>[2x]GKQLTILGSTGSIGCSTLDVVRHNPEHFRVVALVAGKNVTRMVEQCLEFSPRYAVMDDEASAKLLKTMLQQQGSRTEVLSGQQAACDMAALEDVDQVMAAIVGAAGLLPTLAAIRAGKTILLANKESLVTCGRLFMDAVKQSKA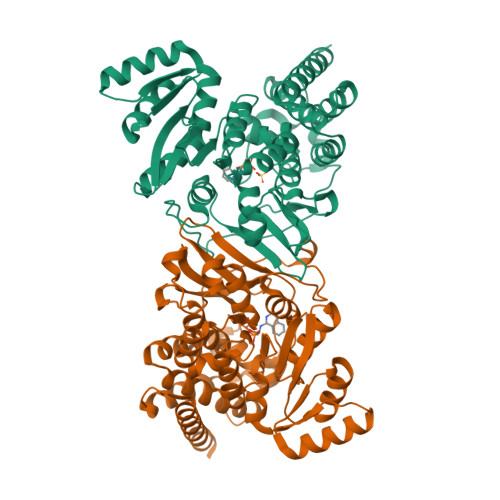QLLPVDSEHNAIFQSLPQPIQHNLGYADLEQNGVVSILLTGSGGPFRETPLRDLATMTPDQACRHPNWSMGRKISVDSATMMNKGLEYIEARWLFNASASQMEVLIHPQSVIHSMVRYQDGSVLAQLGEPDMRTPIAHTMAWPNRVNSGVKPLDFCKLSALTFAAPDYDRYPCLKLAMEAFEQGQAATTALNAANEITVAAFLAQQIRFTDIAALNLSVLEKMDMREPQCVDDVLSVDANAREVARKEVMRLAS> MLHVVQLDDFATRLKAAEDYQSKHSVLSEICDSLETFNAAQDYEYFLKSLIPLFIDVLKEVPVSFVANSPENKLRNITLEILHRIPANDALQAYSNEIVDTLMDLLKVENELNGILCMKAITTLHKTFKASLQEKVHPFIDIVIEIYSNIPQVVEEQFNGNQIDSKENVDSTSRPNSPSFSSQSDDSKQLAQAMFSFKTLAESPITMVSLYSSYKELAASSLGNFIPHVMKVLSLEVAKQAEARKAAEEKGIILVNVCKEITNRANYGEFIIGQVKAASFLAYLFIRRQAQTFLEPYQQAIPDIIIRLLQDCPSELSAARKELLHATRHILSTDFRKMFIPKIDLLFDLRVLIGEGFTAYETLRPLAYSTVADFIHNVRDHLTPAQLWKSVSIYCKNLQDDSLALTVQIMSAKLLLNLIEKIMRSESKTESRQLLMVIIDAYTKRFKMLNSRYNGIMKQHATYEKEKQEKQNQERLLTNKLDGTTPSPSDDKKVELIDEDQDVKMEDPTPEISDQETIKGDNDASTEPQDSEQQLADFMSLQEYLPIQVSVPPEIDLLKDSRYLFKTLMTFLKTIMIGLKNSNPPSSQNHFNAQNWNETARGFSNEDINILKSLFRECILALRFFSTSKTSLPASSMKQSFDITGPNLPITSTKEEKDLMEIFATMFIHIDPASFNEIVREELPFMYKQMLDFASLLHIPQFFLASVITSSSFSGILITFLKSKLVDLGEVNIIKSNILIRLFKLCFMSVSLFPAANESVILPHLNELILKSLKLSTTAKEPLVYFYLIRTLFRSIGGGRFENLYKEIMPLLQVLLESLSKLIHEARRPQERDIYVELCLTVPVRLSVLVPHLSYLMKPLVYALNGSQESVSQGLRTLELCVDNLTAEYFDPIIEPVIDDVMEALSKHLKPLPYYHQHSHTTLRILGKLGGRNRTFIKPVDNLKTDSELFQNVEAMFKIHGLPNEVPLSITPGLSAAFSLLTDPRPRIHYRINSFKYISGIFQLFLGATQLPDDYANRLKESMDIILEDTIAPDEPLNKLHHFPVKDIAKYDSQMELLVKLLESIFYAVSLQEVREESKALIRGTCNHFILLYFNKMVIDKRKFVRKFSVDNHEGNLFLNENCIFDAIIYALSSDNSAVRSMGLESVQLIYDSCVELFGNIDCALKFAPLNVMCSKFIHCCFEEPYHKKLAGCIGLEMMLNSLDIPMKYFNARQLEIIRALFYVLRDTAPELPCEVTNTAKRLILNSLKEWNKELTRNDVFSSVFQNLVSSLIVDLPNANEIVRATAQEALRTLSETTQVPIATMISPCKHILLAPIFGKPLRALPFQMQIGNIDAITFCMGLENSFLEYNEELNRLVQEALALVDAEDESLVSAHRISEHKTSEQLVRLRVVCIQLLSLAITKPEFAAAQQRSNIRVKILVVFFKSLCGRSIEIIRAAHGGLKAVIDLKMKLPKELLQNGLRPMLMNLSDHKKLTVASLEALSGLLKLFISYFKVGIGSKLLDHLLAWAQPRTLQQLGSQDLENNSTVQIIVAILDVFHLLPPTAHKFMNDLMNALLYLENNLHRCQYSPFREPLAKFLDRFPDESFEYFFNEFSKREITTRFVYFVGLDSCSSLRAKVLESLPRVRGLLHQEGSAEEKCVRFSNLVDLCESLAASDKEWIKDKEELLGELLDAGSVCLTLKRSSNVVSPLYFQVDQGFETLQLLYIEYFKSQPLGHEKVFNFIDKISKEGLPFVLEFDDFIFNEVVKCQDIPTVQQTLDTIIRMTPQVSSLDARVYLYKRIFLPICIYESEMHGDLSRLSQTENNELPAWLKSFDSDVWKATGPLVDDYTSTLEDRYRLELMQLTALLIKGAPTALTDMRKDIIKFSWNYIKLDDNTSKQAAYVVTAYFISRFDTPSELTTRIFVALLRCHQIDTRYLVKQALELLAPVLSERTNSELDWLKWPRRVLSEDGFNITQVANIYQLIVKFPDLFYPARDHFIPNIITAMGKLTVMSNTSLENQQLAIDLAELILKWETKLPKSEKLGSAEETEKEKSVSEDKMDIDVKEETKEDIAERPKAEDQIGGDDSDSSNILTSEDYEVSFAQREACVTFLIRYICISTQRPSENELGKRALNILYELLGPKYWSEVTVKLQFFERFLMSSDLNQPSLLGYCLNALEVLAVALKWKPTTWIIENVSYLQKLLEKCLRSDNQDIQEILQKVLGIILEAINKETQGSEEDEPEEVTNFISLIVNIIGEDLSNMTSVAAGVSLCWTLSLYRPNALDSLLPSIMRTFNKLCRDHIAISLQGNQPQSGDFANIEFEAKVTTNLLEKILNLCAARISSLDDQRRVFLSLLAQLIDRSVDKDMLLKVINIVTEWIFKTDFYPTTKEKAGILGKMMIFDLRGEPELSKKFNQVIVDIFESKELAHTELTARMETAFLFGTRLSDVSIRKKLMSILSDSLELDIDKRLFYIIKDQNWEYLSDYPWLNQALQLLYGSFHLDSPIRLSPEENTLSPLQSITEGLAREKSPVEKAPQNIIDFVAKHNEFLDSVRSLTAGDILNPLIDISYQSAETIHNAWVVVFPVAYSAIESRYELEFTRALVKLLFKDYHIRQQDARPNVIKSLLDGVGKCPGLHLPPHLVKYLGSNYNAWYGAIKLLEELSEGQGIDNQKISDANQDALLEVYMSLQEDDMFYGTWRRRAKYFETNAALSYEQIGIWDKALQLYEAAQIKARSGVFPFGESEYSLWEDHWIYCAEKLQHWEILTELAKHEGFTDLLLECGWRGADWIADREPLEQSVKTVMDIPTPRRQIFQTFLALQGFSQQKDTLQDVSRLCDEGIQLTLRKWNALPQRVTRAHIGLLHTFQQYVELMEASQVYSSLVTTNAQNLDVKSQELKRVLQAWRERLPNVWDDINIWNDLVTWRQHVFGVINRVYMPFVPVLQQSNGTNNGNSYAYRGYHEMAWVINRFAHVARKHEMPEVCINQLTKIYTLPNIEIQEAFLKLREQAKCHYQNSSELNTGLDVISNTNLVYFATQQKAEFFTLKGMFLAKLNAKDEANQAFATAVQIDLNLPKAWAEWGFFNDRRFKENPEEIFHAKNAISCYLQAAGLYKDGKTRKLLCRILWLISLDDAAGSLAKTFEDHHGESPVWYWITFVPQLLTSLSHKEAKIVRHILIQIAKSYPQSLHFQLRTTKEDYQAIQRQAMAVNRAEEQSSNKQDTADSVLKNTNTPQPQTRTETSGTTAESDKKPSIPPKEEQGSPQPSRPATTQASPQAQSQENGESSQKHPPEIPTTDSRQPWQDVEEIMGILKTAYPLLALSLESLVDQLNQRFKCNADEDAYRLVIVLYNDGVQQMNRVANPREEVKLPAATEASISRFADSVLPKNIREVFEQDIIACNPNLETYISKLRKWRDCLEEKLDRSYGKADLERVSLHLSLFHHQKFEDIEIPGQYLLHKDNNNHFIKIERFLPTLDLVRGSNGCYKRMTIRGNDGSLHPFAVQFPAARHCRREERIFQLFRIFDDALSRKVQSRRRNISLTLPIAVPLSPHIRILNDDKRYTTLMGIYEEFCRRKGQSRDEPFAYTIQKLRAAFDPRLPKPDIVSVRAEVLASIQSTLVPSTLLKDYYTEKFSNYENYWLFRKQFTAQYASFIFMTYIMCINSRQPQKIHINEGSGNIWTSEMLPTKVATGKTHSTAYNNSTLDPAVKAGAPIFYNTESVPFRLTPNIQKFIGEAGLEGILSVYILVIANSLSDSEFDMEQYLSLFVRDEVISWFAQQHRASAQTNQLREIVRVNVELLTKRVLQLNHIPNSQNVATQFVLNLISQAVNPRNLAYTDSAWMAYL

Here we present the cryo-EM structure of the entire SAGA complex where the major target of activator binding, the 430 kDa Tra1 protein is resolved with an average resolution of 5.7 Å. SAGA is organized into two lobes, one of which is fully occupied by Tra1 while the second contains enzymatic and chromatin recognition functions. The interaction between Tra1 and the second lobe relies on a single and narrow interface forming a hinge region. We find a sequence motif that seems essential for the intricate HEAT domain architecture of Tra1, we identify a structural core shared by other PIKKs including TOR, and we illuminate a resemblance between Tra1 and DNA-PK, a PIKK involved in DNA repair.

While lobe B improved only modestly due to uncorrelated domain movements, the resolution in lobe A reached 5.7 Å, thus showing clear density for helices and several connecting loops. The HEAT repeats form a central solenoid overlaid by a ring structure and adopt a cradle shape when viewed from the side. In agreement with early antibody labeling experiments, the N-terminus of Tra1 is located in a short protruding tail containing 10 α-helices corresponding to residues 1–250. Extending the tail, the central solenoid comprises 11 regular HEAT repeats up to residue 928. These are followed by a linker domain containing three helices before assuming a regular ring-shaped, α-solenoid path, of 31 HEAT repeats. Although the available model of DNA-PK does not contain the full set of HEAT repeats, the comparison with our Tra1 model shows that the overall architecture, shape, and size of the HEAT domain, as well as the positions of the FAT and kinase domains are almost identical. The kinase domain nevertheless maintains the archetypal two-lobe fold of PI3K and the loops that carry the ATP binding residues or the catalytic residues in TOR are located in almost identical positions in Tra1. Strikingly, TOR’s helix Kα9b and the negative regulatory loop sticks into the catalytic cleft and plugs one end of it, while in Tra1 helix Kα9b proceeds in the opposite direction to interact with the FAT domain and there is virtually no analog for the negative regulatory loop. The TRD2 domain in FAT is shifted much closer to the kinase forming new interactions notably with the kinase FATC domain known to be important for Tra1 assembly. Within the shifted TRD2 domain, three consecutive helices that are highly conserved among Tra1 proteins (residues 2698–2753) form a bearing-like module that accepts a rod-shaped density, probably an α-helix, originating from lobe B.Protein tyrosine phosphatases (PTPs) play a critical role in regulating cellular functions by selectively dephosphorylating their substrates. The ∼280 residue PTP catalytic domain consists of an α/β structure, and biochemical and structural studies have led to a detailed understanding of the catalytic mechanism (Barford et al., 1994; Zhang, 2002). Key features of the domain include the PTP signature motif, the mobile Trp-Pro-Asp “WPD” loop that in the closed conformation positions the conserved and catalytically important aspartate residue, and the phosphotyrosine recognition loop. Here we report the crystal structures of 22 PTP domains, including two tandem-domain RPTP structures and a detailed structural comparison of this protein family.

In the second category are PTPs in which both the gateway and the second-site loop are open and accessible as found in the R8 pseudophosphatase group (IA2, IA2β) but a cysteine residue occupies the position of Arg24. Surprisingly, sedimentation velocity measurements showed that all single-domain RPTPs studied (IA2, IA2β, GLEPP1, DEP1, and STEP) were entirely monomeric in solution, as were tandem-domain receptor PTPs (RPTPα, CD45, RPTPɛ, and RPTPμ).

>MSEEPVQSNMDISTGHMILSYMEDHLKNKNRLEKEWEALCAYQAEPNSSFVAQREENVPKNRSLAVLTYDHSRVLLKAENSHSHSDYINASPIMDHDPRNPAYIATQGPLPATVADFWQMVWESGCVVIVMLTPLAENGVRQCYHYWPDEGSNLYHIYEVNLVSEHIWCEDFLVRSFYLKNLQTNETRTVTQFHFLSWYDRGVPSSSRSLLDFRRKVNKCYRGRSCPIIVHCSDGAGRSGTYVLIDMVLNKMAKGAKEIDIAATLEHLRDQRPGMVQTKEQFEFALTAVAEEVNAILAHHHHHH[2x]6-[2-(3-fluoro-5-{2-[(2S)-1-methylpyrrolidin-2-yl]ethyl}phenyl)ethyl]-4-methylpyridin-2-amine 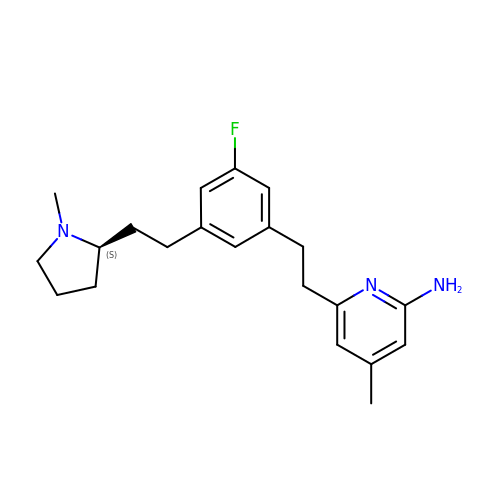| C21 H28 F N3 | LLEZATCTDGWSJC-HXUWFJFHSA-N> MSLVKLMIIEGEVVSGLGEGRYFLSLPPYKEIFKKILGFEPYEGTLNLKLDREFDINKFKYIETEDFEFNGKRFFGVKVLPIKI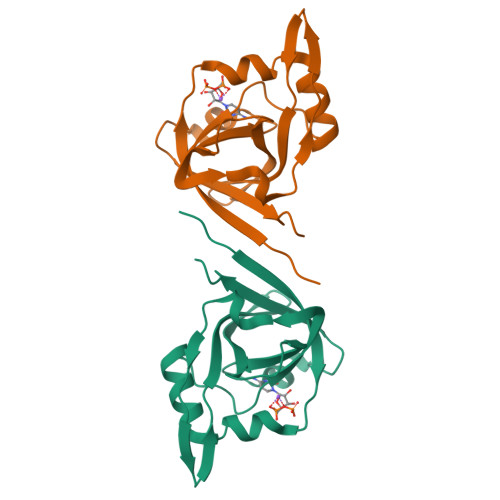LIGNKKIDGAIVVPKKTYHSSEIIEIIAPMKLREQFNLKDGDVIKILIKGDKDEEGHHHHHH> MDKATLVKTIAYRMGNVKGQDTAIDFELALSIERLEGQEFVPWFLLSENNFFEGTAQENRIPVPRGFIREYEEGSLYLRRVAGTGKC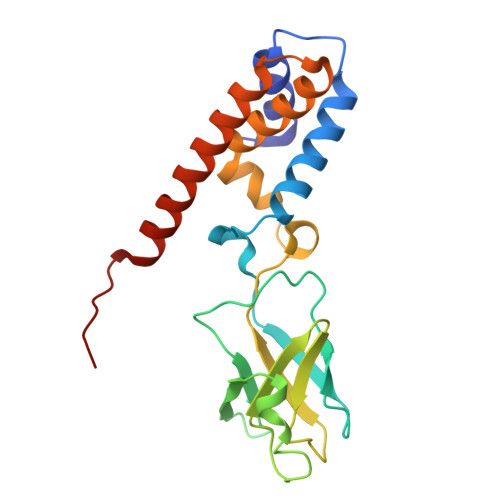LIKKSQDQLLKYEGMTGEPSHYSLTNQYFRIYPVPQEDFKVELLFYRKSSTLNVEDNPWYEYAAELLVAETIWAMLSARRDKMADYWKSVAADQMRRLTILDAERRLANQEIFMG> GAMGEQIFYWSPAKHWRMSDEGVVIGESTYTGMILEWFPEFYFFAQTGVTINRLLERFSSGSEKEANEILELLIQDRVLVEGILPPREVFSPQEGLFVNPYSEQIRYSKEALDYYVSEQLNRTHAAC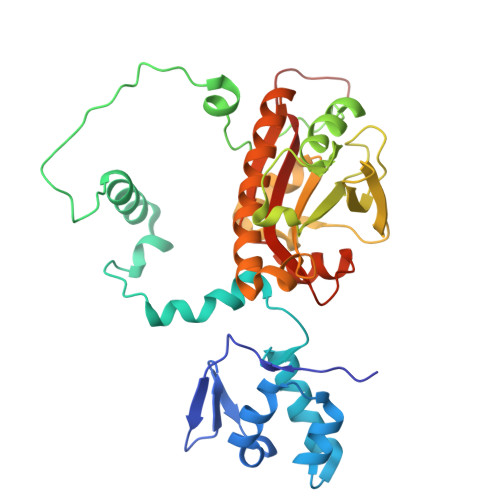RSTKIQLETSGALPDIIQKRRSCRRFDMKTPVSFATFSNLLSSLKQRKEDKILYNYASAGGLYPIDVFVYVKPRRVEGVKAGFYYFNPADHSLVLVNNIDQVIKDDHELINQDIFAQSAFSVYLVYNARASMPKYGAAGYFYACIEAGIITATLNMVAEDLNVGLCSIGHMNFEEIQTFLKLEDHQVILHAIEGGLKIDGAAAENLFY OXA-48 confers resistance to many carbapenem and penicillin β-lactams, but only slowly hydrolyses oxyimino-cephalosporins such as ceftazidime (CAZ). Low catalytic activity for CAZ hydrolysis has been attributed to the substrate’s bulkiness, potentially requiring sampling of alternative loop conformations to promote cephalosporin binding and hydrolysis. Here we reveal how directed evolution of a β-lactamase yielded highly epistatic activity enhancements. We describe how distinct mutations shifted the rate-limiting step from substrate binding to the chemical reaction in the β-lactamase OXA-48, thereby causing strong phenotypic epistasis.

Five mutations accumulated along the evolutionary trajectory, F72L → S212A → T213A → A33V → K51E, resulting in Q5 conferring 43-fold increased CAZ resistance in Escherichia coli. We note that upon CAZ binding in Q5 (Q5-CAZ), the Ω loop becomes highly disordered to the point that it could not be refined anymore, which suggests that incubation with CAZ leads to population of a state that could potentially be less active. To understand how the conformational dynamics affected the substrate-bound state along the evolutionary trajectory, we performed MD simulations of various OXA-48 variants in the acyl–enzyme complex. These models were constructed on the basis of the Q5-CAZ crystal structure with the unresolved Ω loop taken from the apo wtOXA-48 structure. Notably, S212A and T213A enhanced the correlation of S70 with the neighbouring β-strands that harbour the oxyanion hole. This increased correlation could be rooted in the increased rigidification of the β5–β6 loop, harbouring the S212A and T213A mutations, which in turn allows for a tighter interaction of the loop with the substrate.

>[4x]EWQENKSWNVHFTEHKSQGVVVLWNENEQQGFTNNLKRANQAFLPASTLKIPNSLIALDLGVVKDEHQVFKWDGQTRDIATWNRDHNLITAMKYSVVPVYQEFARQIGEARMSKMLHAFDYGNEDISGNVDSFWLDGGIRISATEQISFLRKLYHNKLHVSERSQRIVKQAMLTEANGDYIIRAKTGYAARIEPKIGWWVGWVELDDNVWFFAMNMDMPTSDGLGLRQAITKEVLKQEKIIP>[4x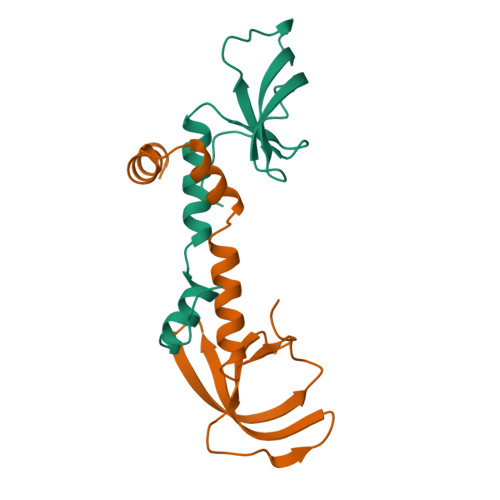]QGPHMDKLAAIKLGRYGEDLLFYLYYMNGGDVLQLLAAVELFNRDWRYHKEERVWITRAPGMEPTMKTNTYERGTYYFFDCLNWRKVAKEFHLEYDKLEERPHLPSTFNYNPAQQAF Site-one protease (S1P, also known as Membrane-bound transcription factor site-1 protease (MBTPS1), or Subtilisin kexin isozyme 1 (SKI-1)), is a membrane-bound protease that mediates the proteolytic activation of transcription factors, hormones, and enzymes required for lipogenesis, the endoplasmic reticulum (ER) stress response, and lysosomal biogenesis, among others. A zymogen serine protease, S1P matures through autoproteolysis of two pro-domains, with one cleavage event in the endoplasmic reticulum (ER) and the other in the Golgi. We recently identified the SREBP regulating gene, (SPRING), which enhances S1P maturation and is necessary for SREBP signaling. SPRING activates S1P by dislodging its inhibitory pro-domain and stabilizing intra-domain contacts.

We therefore obtained a cryo-EM structure of the S1Pecto purified without co-expressed SPRINGecto. The map had a resolution of 2.27 Å using GSFSC cutoff of 0.143 and shows the A-domain bound atop the Peptidase S8 subdomain in a similar position as SPRINGecto. The N- and C-termini of the A-domain run along the side of the Peptidase S8 subdomain. This structure is from a WT S1Pecto sample that has undergone autocatalysis and therefore the density sharply disappears after K137, which corresponds to cleavage at the S1P B-site motif. Our structure of S1Pecto shows that the B-site motif at the C-terminal end of the A-domain is occupying the active site. The P6 Val also makes hydrophobic contacts and the P4 Arg is inserted deeply into an acidic pocket where it makes a salt bridge with D218 of the catalytic triad as well as Q282 and S307. Unlike SPRINGecto, the A-domain of S1Pecto appears to interact only with the Peptidase S8 subdomain. Two loops of the Peptidase S8 subdomain (residues 338-348 and residues 372-384) pack against the GIFT subdomain and were not resolved in the map of S1Pecto without SPRINGecto. Without SPRINGecto, S1Pecto undergoes autocatalysis but remains non-covalently associated with its inhibitory A-domain. Consequently, this S1Pecto is essentially inactive in protease assays based on the S1P cleavage motif from SREBP2.

> METDTLLLWVLLLWVPGSTGDYKDDDDKDRLEKKSFEKAPCPGCSHLTLKVEFSSTVVEYEYIVAFNGYFTAKARNSFISSALKSSEVDNWRIIPRNNPSSDYPSDFEVIQIKEKQKAGLLTLEDHPNIKRVTPQRKVFRSLKYAESDPTVPCNETRWSQKWQSSRPLRRASLSLGSGFWHATGRHSSRRLLRAIPRQVAQTLQADVLWQMGYTGANVRVAVFDTGLSEKHPHFKNVKERTNWTNERTLDDGLGHGTFVAGVIASMRECQGFAPDAELHIFRVFTNNQVSYTSWFLDAFNYAILKKIDVLNLSIGGPDFMDHPFVDKVWELTANNVIMVSAIGNDGPLYGTLNNPADQMDVIGVGGIDFEDNIARFSSRGMTTWELPGGYGRMKPDIVTYGAGVRGSGVKGGCRALSGTSVASPVVAGAVTLLVSTVQKRELVNPASMKQALIASARRLPGVNMFEQGHGKLDLLRAYQILNSYKPQASLSPSYIDLTECPYMWPYCSQPIYYGGMPTVVNVTILNGMGVTGRIVDKPDWQPYLPQNGDNIEVAFSYSSVLWPWSGYLAISISVTKKAASWEGIAQGHVMITVASPAETESKNGAEQTSTVKLPIKVKIIPTPPRSKRVLWDQYHNLRYPPGYFPRDNLRMKNDPLDWNGDHIHTNFRDMYQHLRSMGYFVEVLGAPFTCFDASQYGTLLMVDSEEEYFPEEIAKLRRDVDNGLSLVIFSDWYNTSVMRKVKFYDENTRQWWMPDTGGANIPALNELLSVWNMGFSDGLYEGEFTLANHDMYYASGCSIAKFPEDGVVITQTFKDQGLEVLKQETAVVENVPILGLYQIPAEGGGRIVLYGDSNCLDDSHRQKDCFWLLDALLQYTSYGVTPPSLSHSGNRQRPPSGAGSVTPERMEGNHLHRYSKVLEAHLGDPKPRPLPACPRLSWAKPQPLNETAPSNLWKHQKLLSIDLDKVVLPNFRSNRPQVRPLSPGESGAWDIPGGIMPGRYNQEVHHHHHHHHHH> MK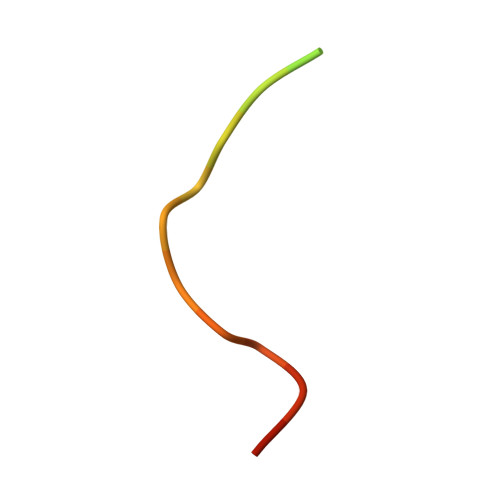RARPSEDTFNPVYPYDTEC N~1~-(3-azaniumylpropyl)butane-1,4-diaminium 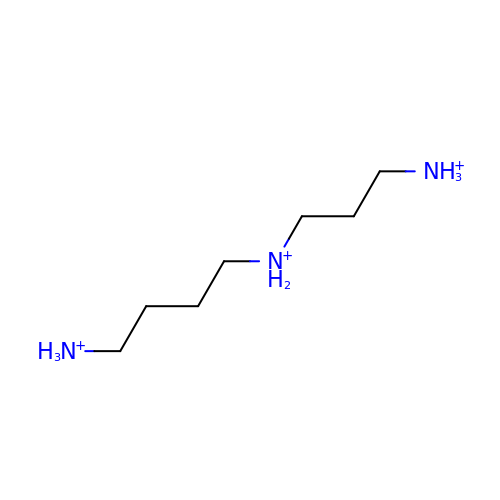| C7 H22 N3 | ATHGHQPFGPMSJY-UHFFFAOYSA-Q Here, we show that the deep neural network ProteinMPNN, together with evolutionary and structural information, provides a route to increasing protein expression, stability, and function. Myoglobin binds heme to carry oxygen in mammalian muscle tissue, and has relevance in clinical applications as a biomarker, as a versatile platform for biocatalytic applications,18−20 and in food science as an ingredient in artificial meat products. Current efforts to create more stable variants of myoglobin have focused on the stabilization of the globin fold through stapling with cysteine-reactive noncanonical amino acids. The globin superfamily, of which myoglobin is a member, has a fold made up of eight alpha helical regions, with diversity in the termini and two loop regions flanking the heme-binding pocket27−29.

To preserve the oxygen storage function, we fixed the identities of 17 positions located around the heme ligand in the heme-bound structure. We selected these less-conserved loop regions for backbone remodeling with RoseTTAFold joint inpainting. We generated two distinct sets of designs with structural remodeling: one with the region joining helices E and F redesigned and one additionally including the CD-loop region. From these remodeled backbones, we again performed sequence design with ProteinMPNN, with the heme-binding site kept fixed. One of the five designs, dnMb19, generated with the more aggressive backbone remodeling strategy, showed a much higher thermal stability of heme binding compared to native myoglobin. We found that it closely agreed with the design model (0.66 Å Cα RMSD), including the regions remodeled with inpainting. Native side chain contacts with the heme group are largely preserved in dnMb19 (inset I). Outside of the heme-binding site, the crystal structure confirms the structural changes introduced by inpainting: the C and E helices were elongated as designed and connected by a new loop (inset II); the loop connecting the E and F helices has a new conformation, and the F helix was straightened through the replacement of PRO88 with GLU89 (inset III). The Cα RMSD over the inpainted regions between the crystal structure and the design model is 0.88 Å, with the largest deviation being in the CD-loop region (1.51 Å). These results illustrate the power of RoseTTAFold joint inpainting and ProteinMPNN to accurately remodel native protein backbones while increasing solubility, thermostability, and functional stability.

>[2x]MSGSEEKAALVLALFDRVEADREEIGAAVLRRTFEEHPETLKKFPRFLELYKKGSPELDALLKEHGKTVLDALIEIARLRYSGEDYRSLIKELAKSHKEEHKIPIEDLRHIAEALLAVLAERFPDEFGPEARAALTDFLDWFIAEIEEEYKKGGGSGSHHWGSTHHHHHH N-[3-(4-chlorophenyl)oxetan-3-yl]-1-propanoyl-1,2,3,4-tetrahydroquinoline-5-carboxamide 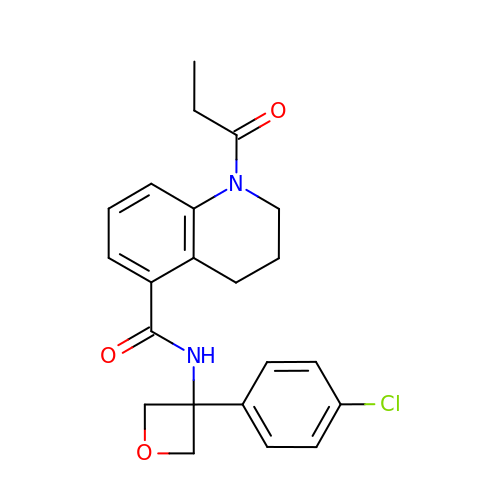| C22 H23 Cl N2 O3 | KBBNTEQRMWVNFG-UHFFFAOYSA-N> MKIDITDYNHADEILNPQLWKEIEETLLKMPLHVKASDQASKVGSLIFDPVGTNQYIKDELVPKHWKNNIPIPKRFDFLGTDIDFGKRDTLVEVQFSNYPFLLNNTVRSELFHKSNMDIDEEGMKVAIIITKGHMFPASNSSLYYEQAQNQLNSLAEYNVFDVPIRLVGLIEDFETDIDIVSTTYADKRYSRTITKRDT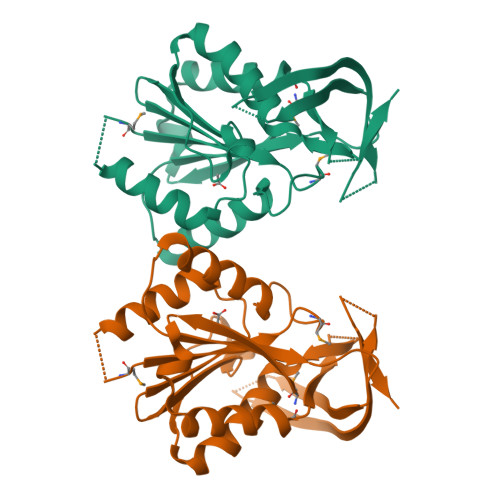VKGKVIDTNTPNTRRRKRGTIVTY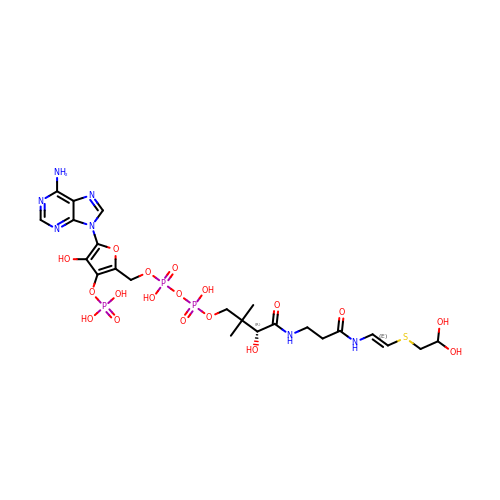[5-(6-amino-9H-purin-9-yl)-4-hydroxy-3-(phosphonooxy)furan-2-yl]methyl (3R)-4-{[3-({(E)-2-[(2,2-dihydroxyethyl)sulfanyl]ethenyl}amino)-3-oxopropyl]amino}-3-hydroxy-2,2-dimethyl-4-oxobutyl dihydrogen diphosphate | C23 H34 N7 O18 P3 S | IWZWXZGRAJOFTE-QWNKOJSDSA-N>[4x]MGHHHHHHMAQKPVDNITQIIGGTPVVKLRNVVDDNAADVYVKLEYQNPGGSVKDRIALAMIEKAEREGKIKPGDTIVEPTSGNTGIGLAFVCAAKGYKAVFTMPETMSQERRNLLKAYGAELVLTPGSEAMKGAIKKAKELKEEHGYFEPQQFENPANPEVHELTTGPELLQQFEGKTIDAFLAGVGTGGTLSGVGKVLKKEYPNIEIV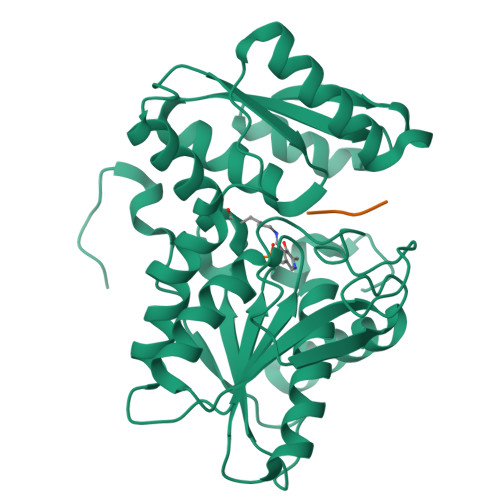AIEPEASPVLSGGEPGPHKLQGLGAGFIPGTLNTEIYDSIIKVGNDTAMEMSRRVAKEEGILAGISSGAAIYAAIQKAKELGKGKTVVTVLPSNGERYLSTPLYSFDD;>[4x]NGEIQDDYII> MDPTTRFRGSDVPVHNEDHMVFAKPSEIGLQGRQGFYTNTNVVTNTYNHVYTPPGGHTGGKFTQDIYTTDLLIAAKDEKADKIPLDKRMDGTFSEGTFVQLLSRGPQDVYLTYNPQISLFKR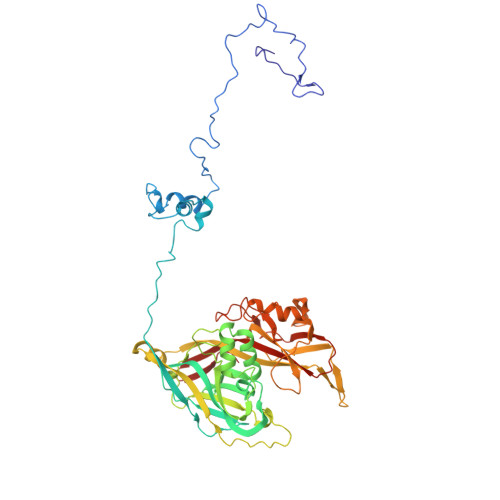KYKRYTNFAIENFEERFSTVVKFGTRNICQLSKNGDLIGNMCFRVTLPNLGIPGGTWAPTMGYNIFSTIRMRIGDTIVQSHDRVWYDIDDKMFCDSTKIQGLDELIKRNVTLTTDQEWELIIPLKFFCCKRNTGKQQFLPILNMDTNINVYLEFNLLPLNSLVTLPTGSILPDIQSIDASVWVDYIFLDDTEKFRFAQDPCVYLIEQTASMDSLSYATTTSGQTYNKTDVYVDMKELNKPVKYVEIIAYEQGSTSFDYVDIIESATFYLNSDEQFKTRAGEYFSLVQPYQHFKRSDPTSNISTFSFALDAGSFQPNGYLNFAPYVRTRFAFKIQPQTTPHVIRLFAVCLNWVKFESGLVKLLFN>GMAESRPARRFARIDRLPPYVFNITAELKMAARRRGEDIIDLSMGNPDGPTPPHIVEKLCTVAQREDTHGYSTSRGIPRLRRAISHWYRDRYDVQIDPESEAIVTIGSKEGLAHLMLATLDHGDTILVPNPSYPIHIYGAVIAGAQVRSVPLVPGIDFFNELERAIRESIPKPRMMILGFPSNPTAQCVELDFFERVVALAKQYDVMVVHDLAYADIVYDGWKAPSIMQVPGAKDIAVEFFTLSKSYNMAGWRIGFMVGNPELVSALARIKSYHDYGTFTPLQVAAIAALEGDQQCVRDIARQYQQRRDVLVKGLREA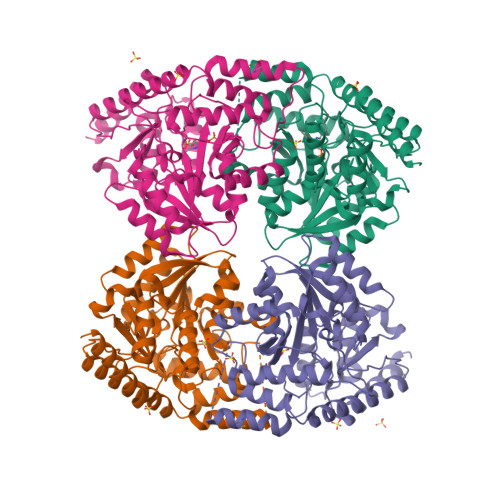GWMVENPKASMYVWAKIPEPYAHLGSLEFAKKLLQDAKVSVSPGIGFGDYGDDHVRFALIENRDRLRQAVRGIKAMFRADGLLSPQRKVDSLAE[4x]>[2x]CUGGGCGG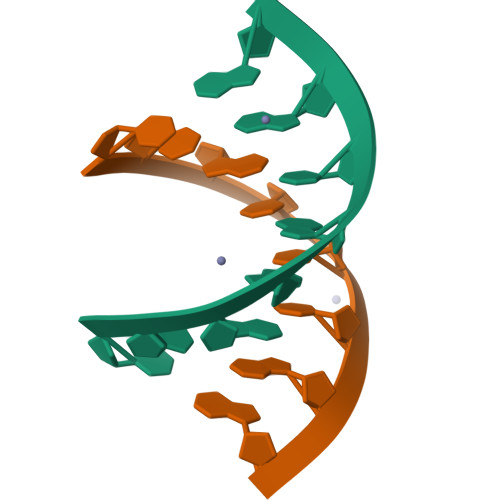;>CCGCCUGG[2x]> SNANINIKKEKVLIPAEVLIQDIPLLKTSFETVRKSRKEIANIIHGNDDRVAVVVGPCSIHDPAAAIEYATKLKEQVKKFHKDILIIMRVYFEKPRTTIGWKGFINDPDLDNSYNINKGLRLARNLLSDLTNMGLPCATEFLDVITPQYFAELITWGAIGARTVESQVHRELASGLSASIGFKNATNGDVQVAVDAVKSATYPHHFLSTTKSGSTAIFATKGNQNGHVILRGGASGPNFSKEHVDDCIAKLKKADINTKVMIDCSHGNSQKDHSKQISVLADICEQIKHSNDIFGVMIESNLVAGNQDINKKPLTYGQSVTDKCVDFEETVKMLEMLAEAVQVRRG

Francisella tularensis, the causative agent of tularemia, is classified by the Centers for Disease Control and Prevention (CDC) as a category A select agent, and its role as a biological weapon is known to have been investigated in the United States, the former Soviet Union, and Japan. Here, we demonstrate how a combined computational and experimental approach based on metabolic network modeling, ligand- and structure-based drug design, physiological modeling, and whole bacterial cell-based assays successfully identified novel antimicrobial compounds in a highly abbreviated time period. Third, we carried out homology modeling and X-ray crystallography to determine the structures of the selected drug targets for subsequent ligand docking. methods, three proteins [3-deoxy-d-arabino-heptulosonate-7-phosphate synthase (aroG), nicotinate-nucleotide pyrophosphorylase (nadC), and d-sedoheptulose 7-phosphate isomerase (lpcA)] were readily crystallized, and their structure was determined using molecular replacement.

We constructed and expressed full-length or slightly shortened recombinant proteins for the remaining targets to optimize protein crystallization without removing any functionally important regions. All structures were prepared as full atomistic models for use in target evaluation and ligand docking. Given computational and experimental limitations on the number of targets and compounds we could screen, we selected a diverse set of 10 candidate targets across a range of metabolic pathways. Our selected targets, as shown in Table 2, included the three enzymes we were able to crystallize (aroG, nadC, and lpcA), four protein homology model structures [shikimate kinase (aroK), pantetheine-phosphate adenylyltransferase (coaD), chorismate synthase (aroC), and 6,7-dimethyl-8-ribityllumazine synthase (ribH)], and three existing PDB crystal structures [enoyl-(acyl carrier protein) reductase (fabI), NAD synthetase (nadE), and 2-amino-4-hydroxy-6-hydroxymethyldihydropteridine pyrophosphokinase (folK)]. The success of generating crystal structures against some of these targets was greatly helped by the availability of genomic DNA, express primer service, and robotics to clone, express, and purify the proteins and to screen crystallization conditions. We mitigated these risks by considering multiple (ten) targets. This proved important because only inhibitors for roughly half the metabolic targets (four) affected bacterial growth in vivo.>MHHHHHHRKAAGKYGNTLEFGHLVGGEEVLEGPLLERRNPSDREDVVARFPEADKDLVRKAALKAREAFAEWSRTPAPIRGQVLFNLVKILEREKPTLTRLMVREVGKTPKEAAGDVQEAIDTALFFASEGRRLYGQTVPSEMRDKELFTFRRPLGVVGIITAGNFPIAVPSWKLIPAVLTGNTVVWKPSEDAPTLSFVFAKLFEEAGLPPGVLNVVFGGGKGSTGQWMVELMDEGLFQKFAFTGSTQVGRWIGEVAGRN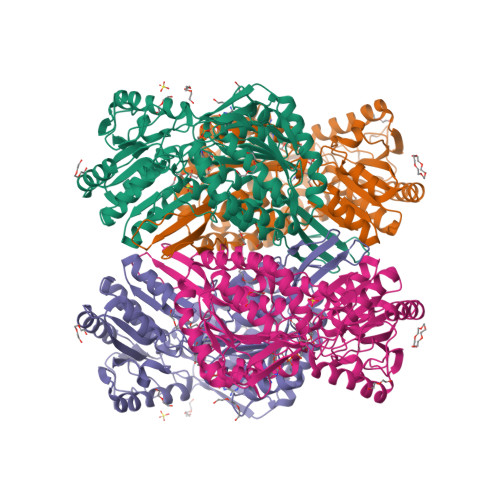LIRPTLELGGKNPLVVMRDADLDLAVEGAWWSAFATGGQRCTSAGNILVDAPIYEEFKRRFLERVEATLVGNPLLHPEVTYGPFINERFFARWQEHYRVGEAEGARLLFGRGRITRENPYPRFLGDPEAGLYGWPTVWEVRPGTRLFTEEVFGPTINLVKVDGIEEAIAVANSTPYGLSSAIYTNHRHWAYLFKVGIRAGMTSINNATVGAEAHLPFGGVKASGNGGRESGIWVLEEYTYWHAVNEEYSGRLQLAQMDTGY[2x]>MPREYEFAEKILFTEEEIRTRIKEVAKRIADDYKGKGLRPYVNPLVLISVLKGSFMFTADLCRALCDFNVPVRMEFICVSSYGEGLTSSGQVRMLLDTRHSIEGHHVLIVEDIVQTALTLNYLYHMYFTRRPASLK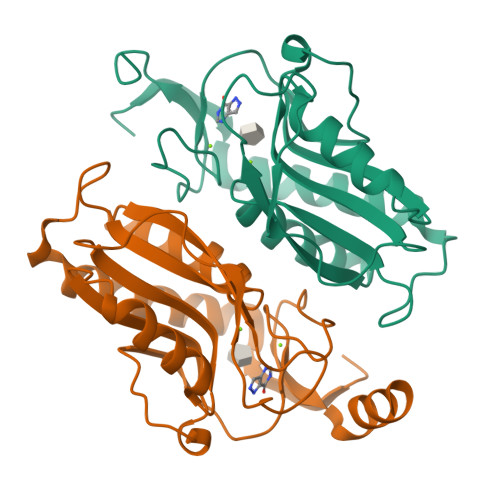TVVLLDKREGRRVPFSADYVVANIPNAFVIGYGLDYDDTYRELRDIVVLRPEVYAEREAARGKKQRAIGSADTDRDAKREFHSKY[2x]> KETAAAKFERQHMDSSTSAASSSNYCNQ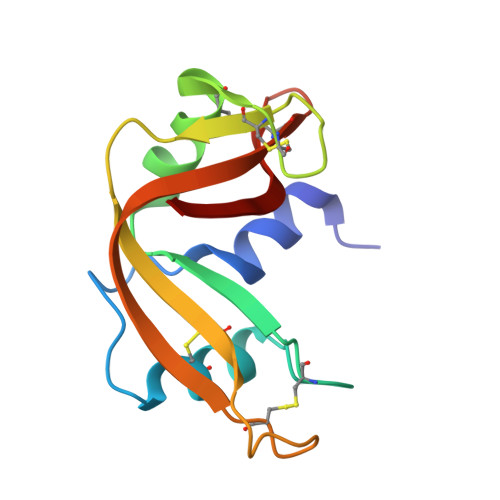MMKSRNLTKDRCKPVNTVVHESLADVQAVCSQKNVACKNGQTNCYQSYSTMSITDCRETGSSKYPNCAYKTTQANKHIIVACEGNPYVPVHFDASV>MPFSDFVLALKDNPYFGAGFGLVGVGTALAMARKGAQLGLVAFRRHYMITLEVPARDRSYAWLLSWLTRHSTRTQHLSVETSYLQHESGRISTKFEFIPSPGNHFIWYQGKWIRVERNRDMQMVDLQTGTPWESVTFTALGTDRKVFFNILEEARALALQQEEGKTVMYTAVGSEWRTFGYPRRRRPLDSVVLQQGLADRIVKDIREFIDNPKWYIDRGIPYRRGYLLYGPPGCGKSSFITALAGELEHSICLLSLTDSSLSDDRLNHLLSVAPQQSLVLLEDVDAAFLSRDLAVENPIKYQGLGRLTFSGLLNALD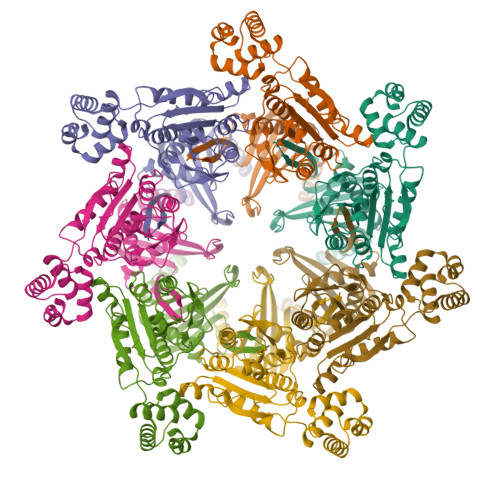GVASTEARIVFMTTNYIDRLDPALIRPGRVDLKEYVGYCSHWQLTQMFQRFYPGQAPSLAENFAEHVLKATSEISPAQVQGYFMLYKNDPMGAVHNIESLRHHHHHH[7x]> MKIAGIDEAGRGPVIGPMVIAAVVVDENSLPKLEELKVRDSKKLTPKRREKLFNEILGVLDDYVILELPPDVIGSREGTLNEFEVENFAKALNSLKVKPDVIYADAADVDEERFARELGERLNFEAEVVAKHKADDIFPVVSAASILAKVTRDRAVEKLKEEYGEIGSGYPSDPR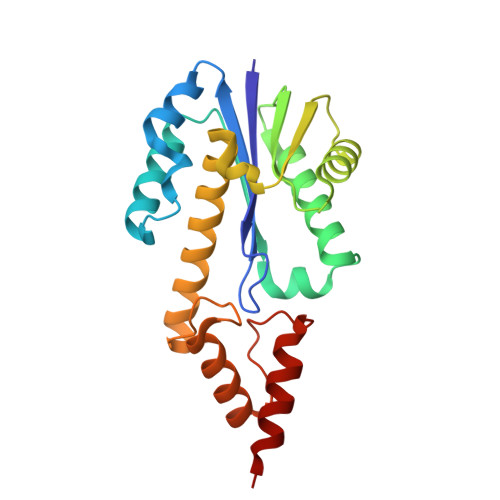TRAFLENYYREHGEFPPIVRKGWKTLKKIAEKVESEKK> GQDRSPIETQNVETVLRLFDEGWGAQDGWRDVWRETMTPGFRSIFHSNQAVEGIEQAIAFNAVLFEGFPRLEVVVENVTVEGDNVVVQARLTGAQDGPFLGVPPSGQMVDVPDVTLFTLADGQVIEMRYF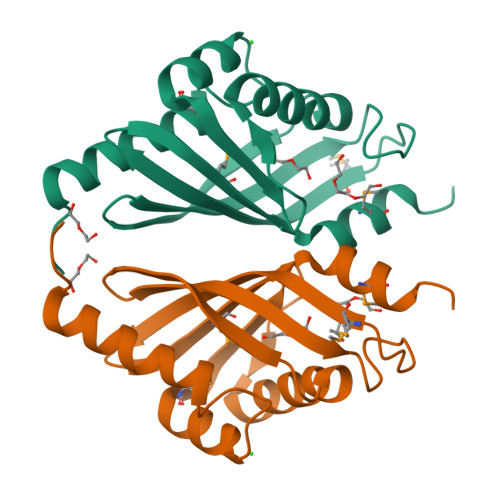TDLLAVMTAISAPPEN>[5x]NNCPLDWLPMNGLCYKIFNQLKTWEDAEMFCRKYKPGCHLASFHRYGESLEIAEYISDYHKGQENVWIGLRDKKKDFSWEWTDRSCTDYLTWDKNQPD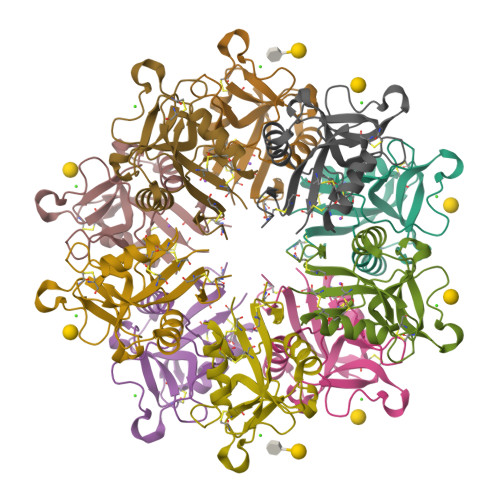HYQNKEFCVELVSLTGYRLWNDQVCESKDAFLCQCKF> QDSTSDLIPAPPLSKVPLQQNFQDNQFHGKWYVVGRAGNTGLREDKDPGKMFATIYELKEDKSYNVTYVWSGQKKCMYSIVTFVPGSQPGEFTLGNIKSAPGRTSWLVRVVSTNYNQHAMVFFK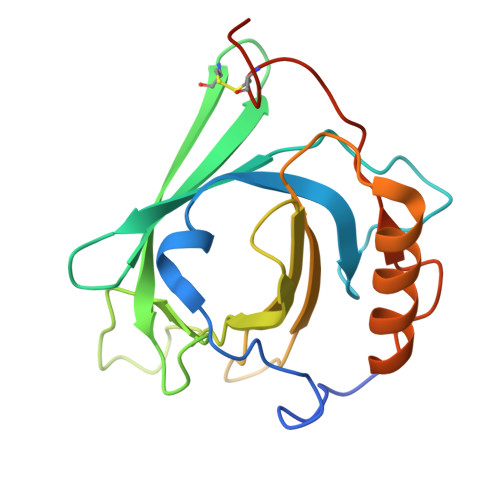SVTQNREGFAITLYGRTKELTSELKENFIRFSKSLGLPENHIVFPVPIDQCIDGSAWSHPQFEK>MYTNSDFVVIKALEDGVNVIGLTRGADTRFHHSEKLDKGEVLIAQFTEHTSAIKVRGKAYIQTRHGVIE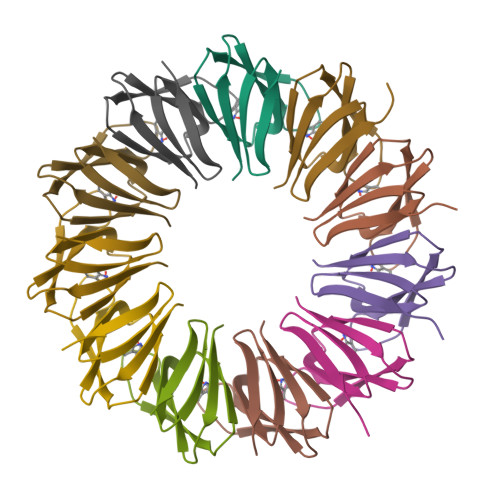SEGKK[11x]> HHHHHHSSGLVPRGSHMQFVNKQFNYKDPVNGVDIAYIKIPNVGQMQPVKAFKIHNKIWVIPERDTFTNPEEGDLNPPPEAKQVPVSYYDSTYLSTDNEKDNYLKGVTKLFERIYSTDLGRMLLTSIVRGIPFWGGSTIDTELKVIDTNCINVIQPDGSYRSEELNLVIIGPSADIIQFECKSFGHEVLNLTRNGYGSTQYIRFSPDFTFGFEESLEVDTNPLLGAGKFATDPAVTLAHELIHAGHRLYGIAINPNRVFKVNTNAYYEMSGLEVSFEELRTFGGHDAKFIDSLQENEFRLYYYNKFKDIASTLNKAKSIVGTTASLQYMKNVFKEKYLLSEDTSGKFSVDKLKFDKLYKMLTEIYTEDNFVKFFKVLNRKTYLNFDKAVFKINIV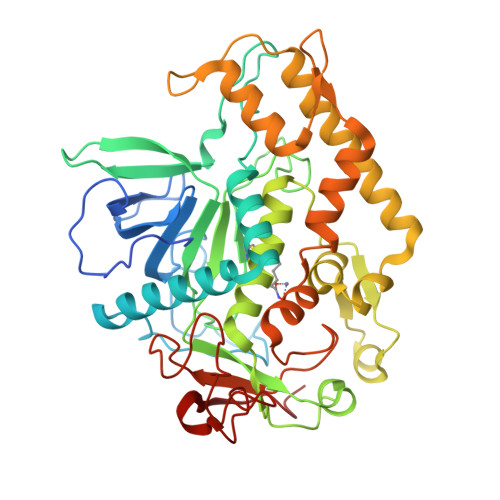PKVNYTIYDGFNLRNTNLAANFNGQNTEINNMNFTKLKNFTGLFE>MGSSHHHHHHSSGRENLYFQGHMKKVVVVGYSGPVNKSPVSELRDICLELGRTLAKKGYLVFNGGRDGVMELVSQGVREAGGTVVGILPDEEAGNPYLSVAVKTGLDFQMRSFVLLRNADVVVSIGGEIGTAIEILGAYALGKPVILL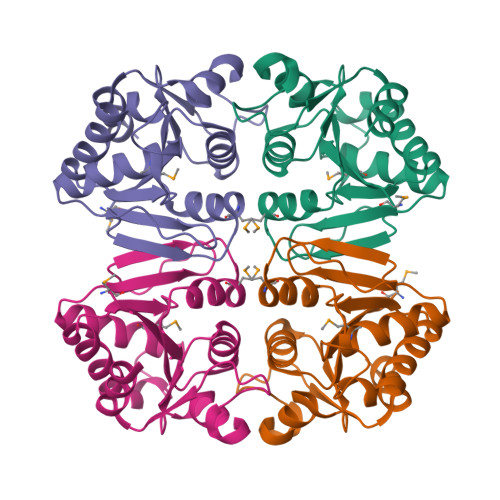RGTGGWTDRISQVLIDGKYLDNRRIVEIHQAWTVEEAVQIIEQILGS[4x]> GSMAWHLGIRSQSRPNDIMAEVCRAIKQLDYEWKVVNPYYLRVRRKNPV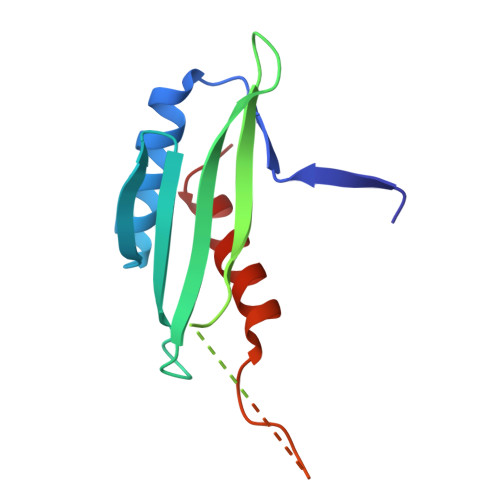TSTFSKMSLQLYQVDSRTYLLDFRSIDDEITEAKSGTATPQRSGSISNYRSCQRSDSDAEAQGKPSEVSLTSSVTSLDSSPVDVAPRPGSHTIEFFEMCANLIKILAQ(2R)-2,3-dihydroxypropyl 2-acetamido-2,4-dideoxy-alpha-L-threo-hex-4-enopyranosiduronic acid | C11 H17 N O8 | 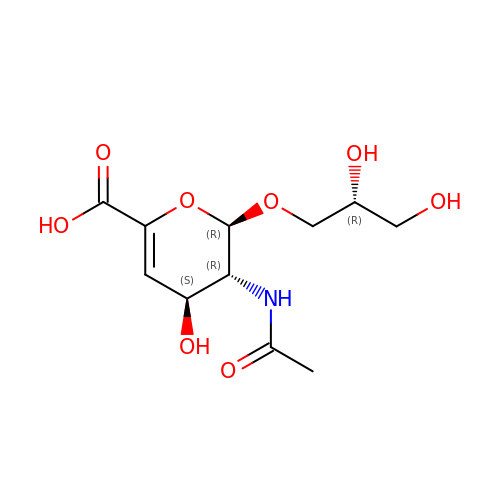HEEZEJCEFZJVGN-YRCORFKGSA-N Transcription in human mitochondria gives rise to two long polycistronic transcripts that are subsequently processed into mature mRNAs, tRNAs and rRNAs by the mitochondrial RNA-processing machinery. According to the tRNA punctuation model, the tRNAs are processed first, and recent work indicates that the primary processing is performed co-transcriptionally through tRNA 5′-processing by mitochondrial RNase P (mt-RNase P). The third subunit, MRPP3 (also known as PRORP: proteinaceous RNase P), contains the sequence features of a zinc-binding domain and an N-terminal, putative RNA-binding pentatricopeptide repeat (PPR) domain, where the PPR repeats are helix-turn-helix motifs of ∼35 amino acids and are found in a large number of RNA binding eukaryotic proteins. Furthermore, the MRPP3 subunit harbors a C-terminal domain that carries the sequence features of a metallonuclease; MRPP3 has therefore been assumed to be the endonucleolytic subunit of mt-RNase P.

Activity assays showed that MRPP3 lacking part of the N-terminal flexible region (Δ102-MRPP3; residues 103–583) was fully active, while removal of the N-terminal flexible region and of PPR motif 1–2 (Δ206-MRPP3; residues 207–583) gives raise to inactive enzyme. Only this inactive construct produced crystals that diffracted to high resolution, which therefore allowed crystal-structure determination. Δ206-MRPP3 is an L-shaped molecule composed of an N-terminal PPR domain, a central domain and a metallonuclease domain. The PPR domain is connected to the metallonuclease domain through the central domain (residues 334–356 and 545–583), which comprises a four-stranded, anti-parallel β-sheet (β1 and β8–10) and harbors the conserved zinc-binding site. A long loop region between β9 and β10 (hereafter referred to as the lariat loop; residues 560–575) intercalates between the metallonuclease and PPR domains. When comparing the structure of this region in Δ206-MRPP3 and the homologous PRORP1, it becomes clear that the Δ206-MRPP3 active site is distinctly different from that of PRORP1. In human Δ206-MRPP3, however, the equivalent residue to N492P is R498, which occupies the metal-binding site, and forms a salt bridge with D478. At the same time, D499 is flipped out of the active site to hydrogen bond with the S569 of the lariat loop. The first key difference between Δ206-MRPP3 and PRORP1 is that the individual domains are oriented differently. Δ206-MRPP3 adopts a relaxed, twisted, L-shaped conformation with the metallonuclease domain being moved out of the plane formed by the PPR and the central domains. We propose that MRPP3 is kept in a non-productive conformation by a dual-control mechanism, namely by the presence of a non-productive active site and by the orientation of the individual domains toward each other.

> SMTLEPRGYSLLIRGLIHSDRWREALLLLEDIKKVITPSKKNYNDCIQGALLHQDVNTAWNLYQELLGHDIVPMLETLKAFFDFGKDIKDDNYSNKLLDILSYLRNNQLYPGESFAHSIKTWFESVPGKQWKGQFTTVRKSGQCSGCGKTIESIQLSPEEYECLKGKIMRDVIDGGDQYRKTTPQELKRFENFIKSRPPFDVVIDGLNVAKMFPKVRESQLLLNVVSQLAKRNLRLLVLGRKHMLRRSSQWSRDEMEEVQKQASCFFADDISEDDPFLLYATLHSGNHCRFITRDLMRDHKACLPDAKTQRLFFKWQQGHQLAIVNRFPGSKLTFQRILSYDTVVQTTGDSWHIPYDEDLVERCSCEVPTKWLCLHQKT> MASTTRLVNDRKQLEQQVKDDARILADARGLNITTVANDSATGGQAIRNVGPNDEATIKALDNVIKQIEALSVIVNRSEKADDAQILGPNTYKQLLEHLFSPEENVYILLPIQAYTGGVIDRRDASFSNFAYSIASKLMMELSAATHNKIFTDYTRIAASALGPEISTEGMPLFSLIESLELTEAETSRLPVIQDSMVIQKSTATVGNAQQGISTINIKRVPFVGSAFQQVIDQLLWEYSTTSLTTKEQRRQRITEMVNDRRIMIQKLTLAEKPQVMRHVTTEINNDLFFKMSPVAQLYIYHLDRAFLDGVGFTPLAEKQQQLQLQLKTNILTANLIRSAINGMNTESNLEVAIKMMQAAQLHRASIEIAFPMNVSLSPEIIVQCFIVWMSIPEQLLSDRSNFIIAAVIWAGFSADDSYADIMRRSARASDRQNYDIIKAALSSRKFKLPRASTTLFDENEPVVRRYQIGRVYAPFPVDRYGSPVYSNCTKVELASDYNAEGFTIRKDDFRALQAVLRIDEDRAADMFTTLRIMISSIPAVWYDAEVVHYPHTAVELEQLAAYGLTGAYPRTNHSVDTIVKTVNNISATYSTIAQMLSTIDLDPTRYGTSESIDKFKIAWENVESVLNMEGNDFVKTIMYAYEDNFPKKDFYMMLKQIASDGQGAHPIAAAIDQLRTIVYREPERF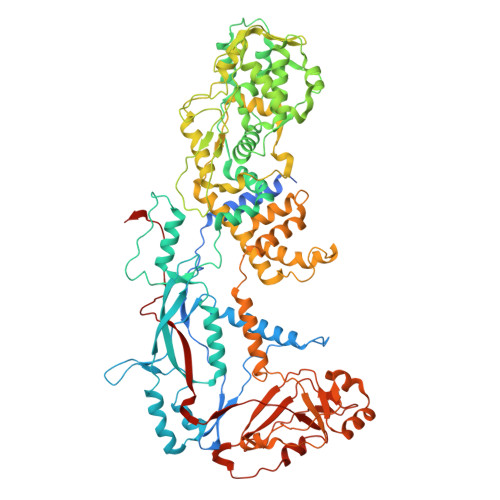GYIDSVILTHNPDVDTAYNRFFHLHPIVTNQPSNTIKNAQLWNEMRLEQQVEHIKAGPVRIIGPFHVTYNYLSEEEDMPATSHIIMKDNMILNDHLTFNFVKRERRNNKKRVSSFRYKAVEMYVAVRISRFQLEVLRDLHDLVRSRTYLDVSKSPLATTPIRVVEYVR> APYASLTEIEHLVQSVCKSYRETCQLRLEDLLRQRSNIFSREEVTGYQRKSMWEMWERCAHHLTEAIQYVVEFAKRLSGFMELCQNDQIV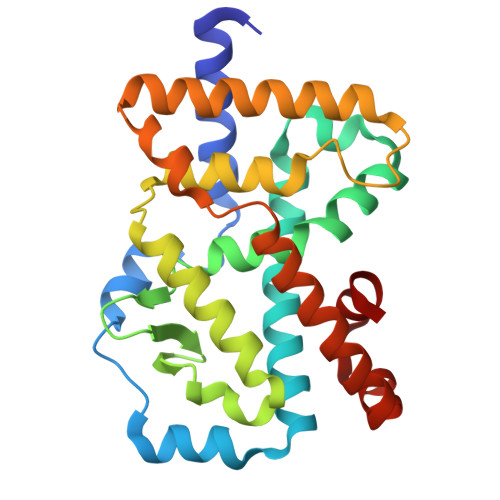LLKAGAMEVVLVRMCRAYNADNRTVFFEGKYGGMELFRALGCSELISSIFDFSHSLSALHFSEDEIALYTALVLINAHRPGLQEKRKVEQLQYNLELAFHHHLCKTHRQSILAKLPPKGKLRSLCSQHVERLQIFQHLHPIVVQAAFPPLYKELFS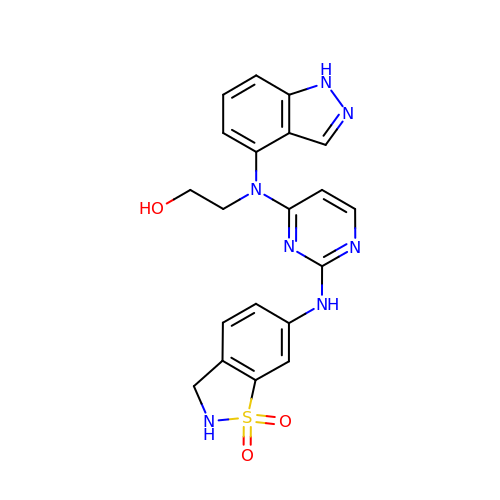2-[{2-[(1,1-dioxido-2,3-dihydro-1,2-benzothiazol-6-yl)amino]pyrimidin-4-yl}(1H-indazol-4-yl)amino]ethanol | C20 H19 N7 O3 S | FJNNGDRUSXSMAJ-UHFFFAOYSA-N>[2x]GPGSMAQLKGSKTEENLKYAFAGESQANRRYLYFASKADVEGQNDIA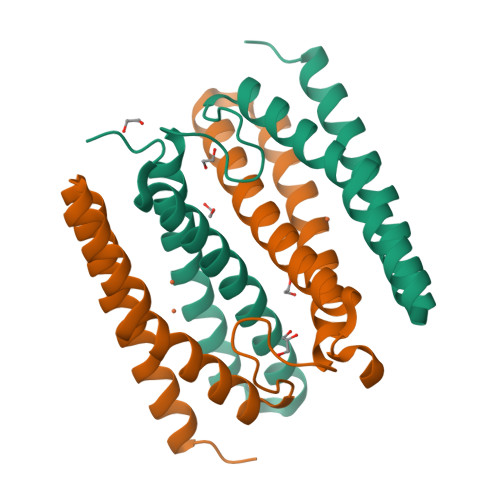ALFRSTAEGETGHAHGHLEYLEAVGDPATGLPFGTSRQNLQSAIAGETHEYTDMYPGMAKTARDEGFEEIANWFETLAKAERSHANRYTKALDGLVD>MAPKQTPSPEKNRNLVGPVLQRRQTEGTFDQRLLEMRADHNWKHADPWRVLRIQSEFVAGFDALHEMPKAVTVFGSARIKEDHPYYKAGVELGEKLVAADYAVVTGGGPGLMEAPNKGASEANGLSVGLGIELPHEQHLNPYVDLGLNFRYFFARKTMFLKYSQAFVCLPGGFGTLDELFEVLCMVQTGKVTNFPIVLIGTEFWAGLVDWIRHRLVEEGMIDEKDVDRMLVTDDLDQAVKFIVDAHAGLDVARRHNLEHHHHHH[3x]

In cytokinin biosynthesis, the Lonely Guy (LOG) protein has been recently identified as a phosphoribohydrolase that finally releases cytokinins. LOG proteins produce active cytokinins via dephosphoribosylation, directly hydrolyzing the bond between N6-substituted bases and ribose 5′-monophosphates in conjugated forms. Based on the biochemical and in vivo cytokinin production experiments, we propose that Cg1261 is a novel type of LOG and belongs to type II LOGs (CgLOGII). Comparative analysis of 123 LOG-like proteins also suggested that LOG proteins could be divided into two different types, dimeric type I LOGs and hexameric type II LOGs.

To investigate the function of Cg1261, we determined its crystal structure at a resolution of 1.95 Å and revealed its hexameric oligomerization involving the extended N-terminal region. The asymmetric unit contained three molecules (Molecules I, II, and III), and the crystal volume per unit of protein mass was approximately 1.91 Å3·Da−1, which corresponds to a solvent content of approximately 35.76%. Interestingly, the electron density maps of the N-terminal region (Met1–His39) were invisible in all three molecules, indicating that this region is highly disordered (hereinafter referred to as disordered N-terminal region, DNR). The Cg1261 monomer forms a Rossmann α/β structure and is composed of eight α-helices and seven parallel β-strands. Molecules I and II form a dimeric structure, which is similar to the dimeric structure of CgLOG. The hexameric structure was formed by oligomerization of three dimeric structures, and the overall shape of the hexamer looked like a trillium flower, in which each petal was made up of a twisted dimer. The α1 helices of six monomers mainly contribute to hexamerization of Cg1261. Compared with CgLOG, Cg1261 contained an extended N-terminal region, which formed an α1 helix (Asp46–Leu64). Two catalytic residues, Arg155 and Glu178, are located near the covalent bond between adenine-N9 and ribose-C1, which is hydrolyzed by the enzyme.>[2x]MQNITQSWFVQGMIKATTDAWLKGWDERNGGNLTLRLDDADIAPYHDNFHQQPRYIPLSQPMPLLANTPFIVTGSGKFFRNVQLDPAANLGIVKVDSDGAGYHILWGLTNEAVPTSELPAHFLSHCERIKATNGKDRVIMHCHATNLIALTYVLENDTAVFTRQLWEGSTECLVVFPDGVGILPWMVPGTDAIGQATAQEMQKHSLVLWPF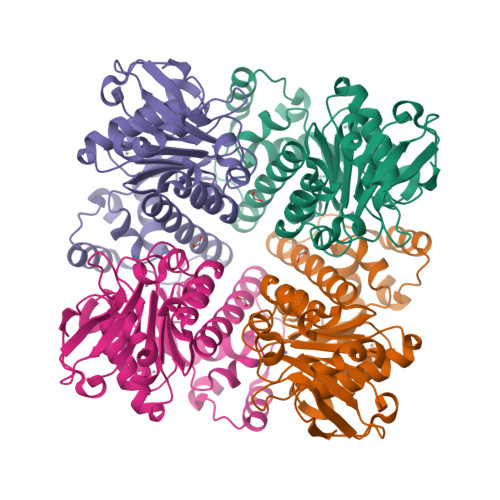HGVFGSGPTLDETFGLIDTAEKSAQVLVKVYSMGGMWQTISREELIALGKRFGVTPLASALA>QTPTGIYYEVRGDTIYMINVTSGEETPIHLFGVNWFGFETCNHVVHGLWKRNWEDMLLQIKSLGFNAIR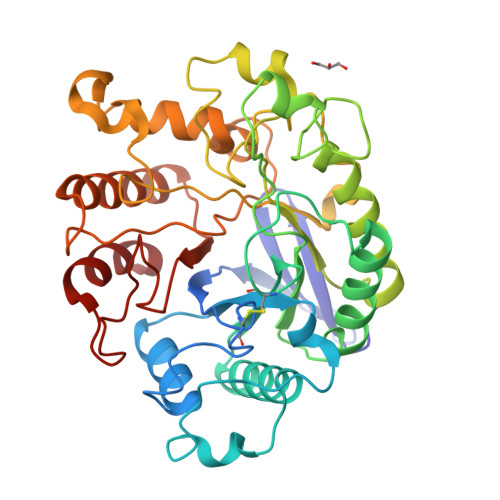LPFCTESVKPGTQPIGIDYSKNPDLRGLDSLQIMEKIIKKAGDLGIFVLLDYHRIGCTHIEPLWYTEDFSEEDFINTWIEVAKRFGKYWNVIGADLKNEPHSVTSPPAAYTDGTGATWGMGNPATDWNLAAERIGKAILKVAPHWLIFVEGTQFTNPKTDSSYKWGYNAWWGGNLMAVKDYPVNLPKNKLVYSPHVYGPDVYNQPYFGPAKGFPDNLPDIWYHHFGYVKLELGYSVVIGEFGGKYGHGGDPRDVIWQNKLVDWMIENKFCDFFYWSWNPDSGDTGGILQDDWTTIWEDKYNNLKRLMD[3x]> AESTLGAAAAQSGRYFGTAIASGRLSDSTYTSIAGREFNMVTAENEMKIDATEPQRGQFNFSSADRVYNWAVQNGKQVRGHTLAWHSQQPGWMQSLSGSALRQAMIDHINGVMAHYKGKIVQWDVVNEAFADGSSGARRDSNLQRSGNDWIEVAFRTARAADPSAKLCYNDYNVENWTWAKTQAMYNMVRDFKQRGVPIDCVGFQSHFNSGSPYNSNFRTTLQNFAALGVDV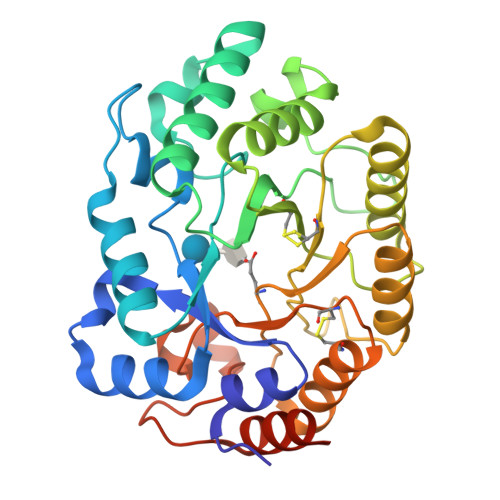AITELDIQGAPASTYANVTNDCLAVSRCLGITVWGVRDSDSWRSEQTPLLFNNDGSKKAAYTAVLDALNGGASSEPPADGG>AGGGAGGGCGCTGGGAGGA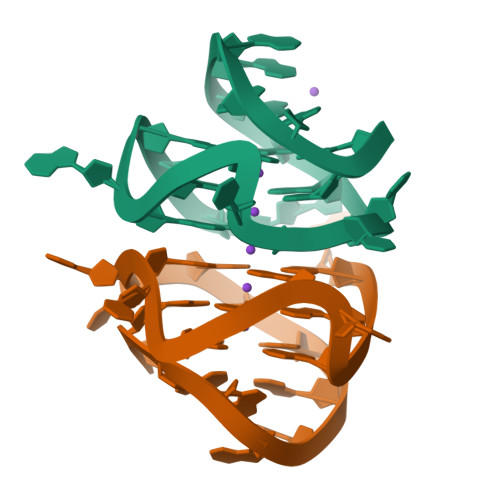GGG[2x]> ADPLLPYFDFDVPRNLTVTVGQTGFLHCRVE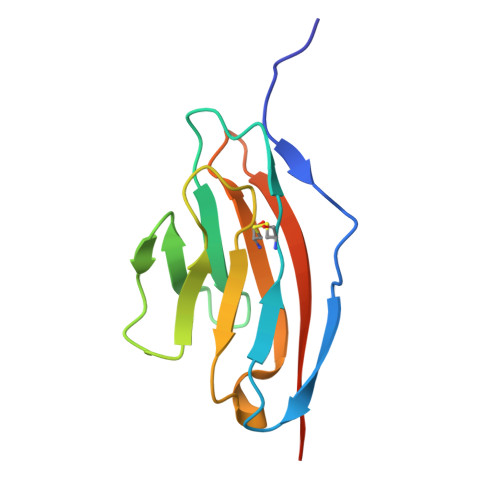RLGDKDVSWIRKRDLHILTAGGTTYTSDQRFQVLRPDGSANWTLQIKYPQPRDSGVYECQINTEPKMSLSYTFNVVEHHHHHH>MAIITPALISALKTSFQKHFQDALATAPSTYLQVATVIPSTTASNTYGWLGQFPKLREWIGQRVIKDMAAQGYQITNKLFESTVGVKRTDIEDDNLGVYGPLMQEMGRAAGAHPDELVFALLKAGNANLCYDGQNFFDTDHPVYPNVDGTGTATTVSNLFAPAADPGAAWYLLDTSRSLKPLIYQERMKPSFTSMTKEDDEQVFMADEYRYGVRSRCNVGFGFWQLAAMSTEELNQVNFEKVYDAMRNQKADGGRPLDIRPNLLVVPTTLRSKAKEVVGVQRLANGADNPN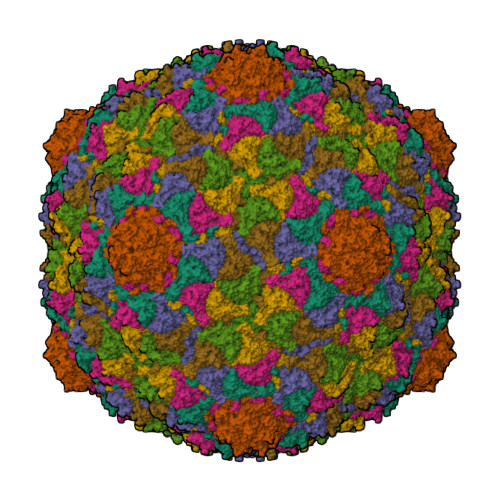FELVQVLDTAWLN[7x]PHENYL DIHYDROGEN PHOSPHATE | C6 H7 O4 P | 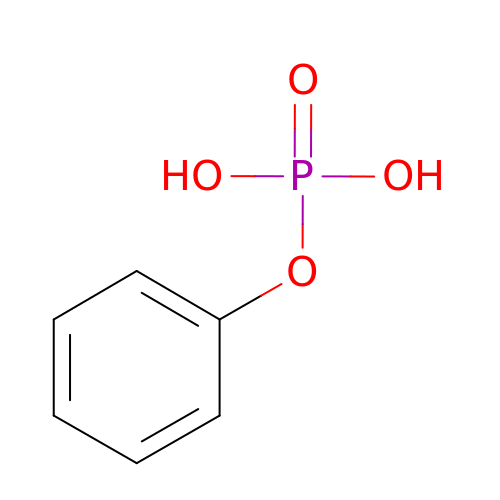CMPQUABWPXYYSH-UHFFFAOYSA-N>[2x]MKTKKHALLFAALLLGGMSASYALEMTGLKPGVPASTATAQAMAKRHATLYGDPAGQSQASRIIDVKPGMRYVNVDSGETVAFRAGEKIVAWTFAQMVRDTSVDLGL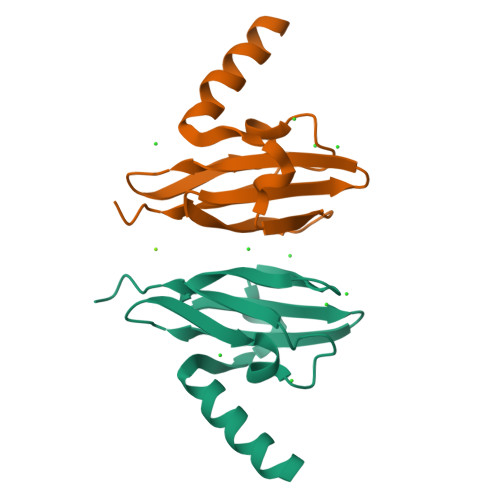LMPDLPGSAGVRVYIDRSDLFTGG> AMADIGSMNLNSIPAFQDNYIWVLTNDEGRCVIVDPGEAAPVLKAIAEHKWMPEAI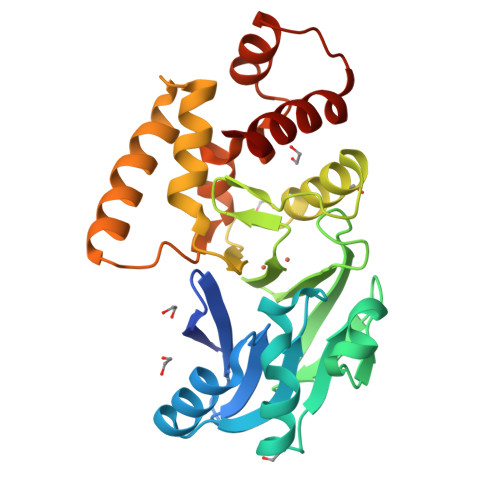FLTHHHHDHVGGVKELLQHFPQMTVYGPAETQDKGATHLVGDGDTIRVLGEKFTLFATPGHTLGHVCYFSRPYLFCGDTLFSGGCGRLFEGTPSQMYQSLMKINSLPDDTLICCAHEYTLANIKFALSILPHDSFINEYYRKVKELRVKKQMTLPVILKNERKINLFLRTEDIDLINEINKETILQQPEARFAWLRSKKDTF>[4x]MRSRRVDVMDVMNRLILAMDLMNRDDALRVTGEVREYIDTVKIGYPLVLSEGMDIIAEFRKRFGCRIIANFKVADIPETNEKIC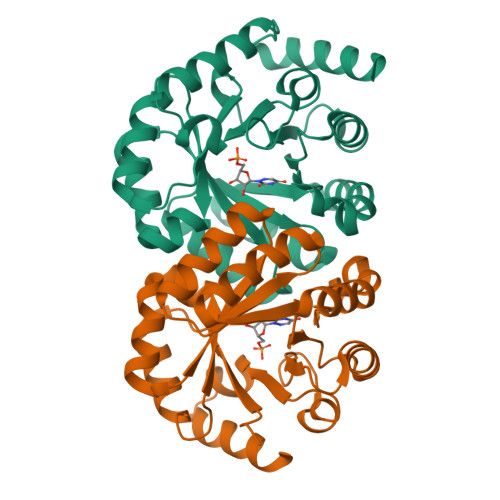RATFKAGADAIIVHGFPGADSVRACLNVAEEMGREVFLLTEMSHPGAEMFIQGAADEIARMGVDLGVKNYVGPSTRPERLSRLREIIGQDSFLISPGVGAQGGDPGETLRFADAIIVGRSIYLADNPAAAAAGIIESIKDLLIPEDPAANKARKEAELAAATA> MTLLSPGIELKETTVQSTVVNNSTGTAALAGKFQWGPAFQIKQVTNEVDLVNTFGQPTAETADYFMSAMNFLQYGNDLRVVRAVDRDTAKNSSPIAGNIEYTISTPGSNYAVGDKITVKY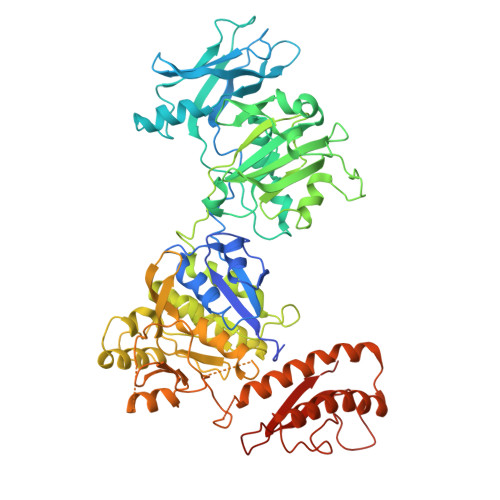VSDDIETEGKITEVDADGKIKKINIPTAKIIAKAKEVGEYPTLGSNWTAEISSSSSGLAAVITLGKIITDSGILLAEIENAEAAMTAVDFQANLKKYGIPGVVALYPGELGDKIEIEIVSKADYAKGASALLPIYPGGGTRASTAKAVFGYGPQTDSQYAIIVRRNDAIVQSVVLSTKRGGKDIYDSNIYIDDFFAKGGSEYIFATAQNWPEGFSGILTLSGGLSSNAEVTAGDLMEAWDFFADRESVDVQLFIAGSCAGESLETASTVQKHVVSIGDVRQDCLVLCSPPRETVVGIPVTRAVDNLVNWRTAAGSYTDNNFNISSTYAAIDGNYKYQYDKYNDVNRWVPLAADIAGLCARTDNVSQTWMSPAGYNRGQILNVIKLAIETPQAQRDRLYQEAINPVTGTGGDGYVLYGDKTATSVPSPFDRINVRRLFNMLKTNIGRSSKYRLFELNNAFTRSSFRTETAQYLQGNKALGGIYEYRVVCDTTNNTPSVIDRNEFVATFYIQPARSINYITLNFVATATGADFDELTGLAG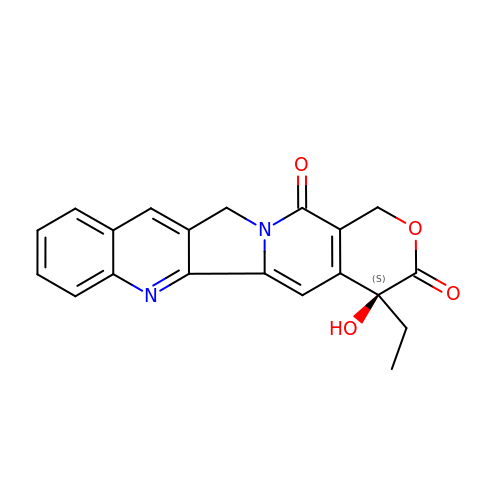4-ETHYL-4-HYDROXY-1,12-DIHYDRO-4H-2-OXA-6,12A-DIAZA-DIBENZO[B,H]FLUORENE-3,13-DIONE | C20 H16 N2 O4 | VSJKWCGYPAHWDS-FQEVSTJZSA-N> ETMSGPLHIGLIPTVGPYLLPHIIPMLHQTFPKLEMYLHEAQTHQLLAQLDSGKLDAVILALV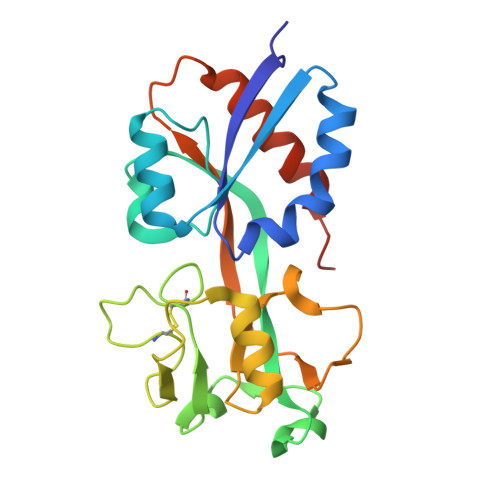KESEAFIEVPLFDEPMLLAIYEDHPWANREAVPMADLAGEKLLMLEDGHCLRDQAMGFCFEAGADEDTHFRATSLETLRNMVAAGSGITLLPALAVPPERKRDGVVYLPAIKPEPRRTIGLVYRPGSPLRSRYEQLAEAIRARMDGHFDKVLKQAV> SGTATYSGNPFVGVTPWANAYYASEVSSLAIPSLTGAMATAAAAVAKVPSFMWLDTLDKTPLMEQTLADIRTANKNGGNYAGQFVVYDLPDRDCAALASNGEYSIADGGVAKYKNYIDTIRQIVVEYSDIRTLLVIEPDSLANLVTNLGTPKCANAQSAYLECINYAVTQLNLPNVAMYLDAGHAGWLGWPANQDPAAQLFANVYKNASSPRALRGLATNVANYNGWNITSPPSYTQGNAVYNEKLYIHAIGPLLANHGWSNAFFITDQGRSGKQPTGQQQWGDWCNVIGTGFGIRPSANTGDS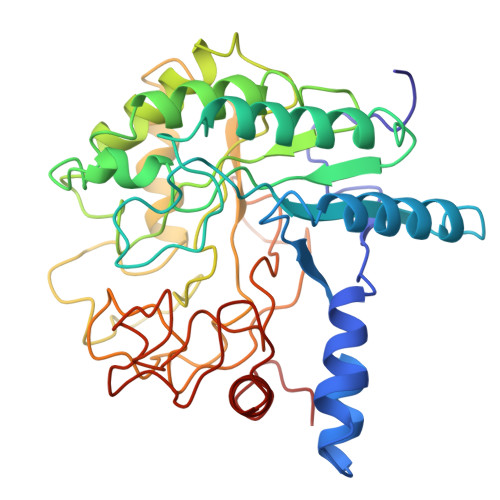LLDSFVWVKPGGECDGTSDSSAPRFDSHCALPDALQPAPQAGAWFQAYFVQLLTNANPSFL>[14x]XGEIAKALREIAKALREIAWA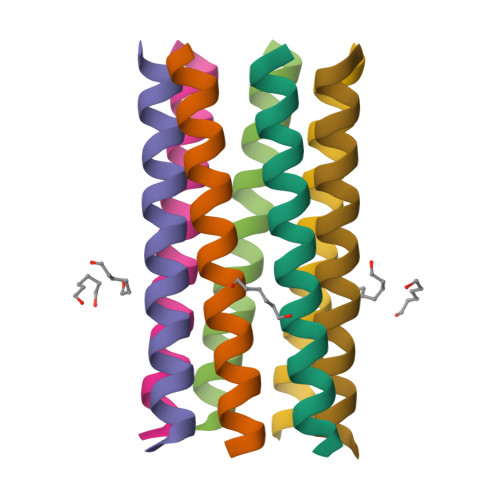NRENAKALRGX3-[(5-{[3-(2,6-dichlorophenyl)-5-(1-methylethyl)isoxazol-4-yl]methoxy}-1H-indol-1-yl)methyl]benzoic acid | C29 H24 Cl2 N2 O4 | 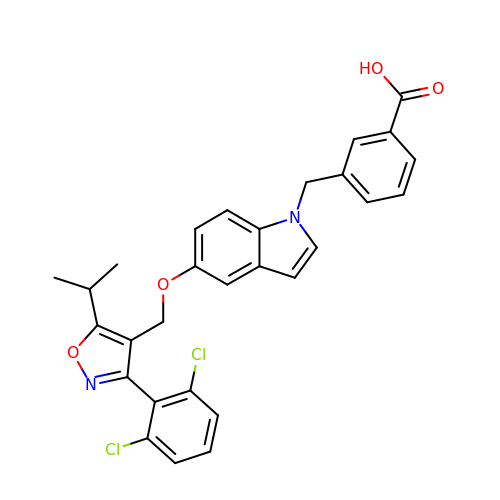FCSGTZIUJUNGAC-UHFFFAOYSA-N>EAGITGTWYNQLGSTFIVTAGADGALTGTYESAVGNAESRYVLTGRYDSAPATDGSGTALGWTVAWKNNYRNAHSATTWSGQYVGGAEARINTQWLLT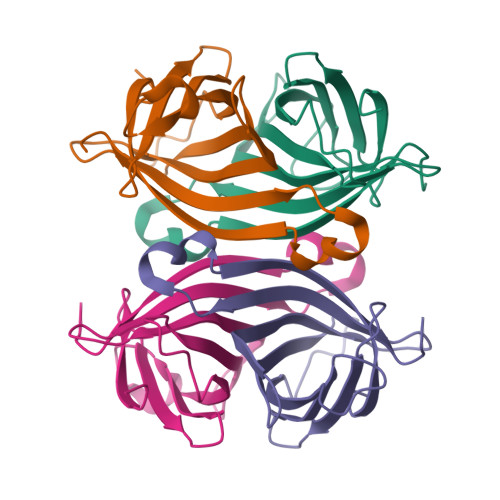SGTTEANAWKSTLVGHDTFTKVKPS[4x]> MDNKPETSLDNPVHQRSEPGSETGSSLSTITTHHLTVPPGLTPEEFQELSSSIAEFHSYRINPGQCSSLLAQRIHAPVETVWTVVRRFDKPQTYKHFIKSCSVGEDFRMTVGSTRDVTVISGLPAATSTERLDILDDDRHVTGFSIIGGEHRLRNYRSVTTVHGFERDGEIWTVVLESYVVDVPEGNTEEDTRLFADTV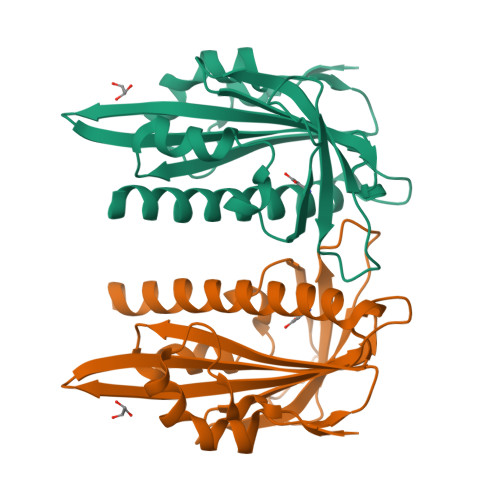VKLNLQKLASVTETLAREAGNGSVNSRDASHRS> GAGCAGACGTGGAGCAGACGTG;> ACCCCACTCA;> CAGGT;> TCTGAGTGGCGTCTGC

In this work, we exhaustively probe the ability of all 36 immobile HJ sequences to form DNA crystals in two different designed systems. Three separate self-assembling DNA crystal systems are described in this report: the “4 × 5” and “4 × 6” designs (collectively referred to as the 4 × N systems), and a third construct with a “scrambled” sequence variant of the 4 × 6 lattices. Self-assembly was mediated by three constituent oligonucleotides: (S1) containing four sequence repeats of either 5 or 6 bases; (S2) composed of 21 bases containing complementary regions to both (S1); and (S3) which forms the second junction crossover. The HJ serves as the fundamental component at the core of each unit, and the ultimate assembly of the full lattice is facilitated by the complementary 2-base sticky ends that tail each duplex.

The 4 × 5 system robustly crystallized with 75% of the junctions, and we obtained crystals in all but 9 of 36 sequences. Of the resulting structures, 18 exhibited P32 symmetry with average cell dimensions a = b = 68.85 Å c = 60.09 Å, with only nine retaining the original P3221 symmetry with average cell edges a = b = 68.17 Å c = 60.60 Å. Although the cell parameters between the two symmetries were virtually indistinguishable, the differences between the periodicity of the lattices is dramatic, with vastly different cavity sizes. While the highest resolution achieved for the J1 system was 3.1 Å, in roughly half of the crystals measured the resolutions were 3.05 Å or better, and as high as 2.9 Å (J6) and 2.75 Å (J19), for the P32 and P3221 symmetries, respectively. Pos1 and 2 were readily observable in the electron density maps at either one or both of these conserved sites in a significant number of the structures, with no apparent respect to motif or symmetry. However, in the majority of the crystal structures reported here, the cacodylate anion indeed fits best into the electron density map of our X-ray structures, due to the presence of sodium cacodylate in the crystallization solution.> GPLGSGGGTIAMLNEISSDTLEQLYSLAFNQYQSGKYEDAHKVFQALCVLDHYDSRFFLGLGACRQAMGQYDLAIHSYSYGAVMDIKEPRFPFHAAECLLQKGELAEAESGLFLAQELIANKPEFKELSTRVSSMLEAIKLKKEMKHE;> XQVPELIKPSQ

SycD (specific Yop chaperone D) from the enteropathogen Yersinia enterocolitica is the class II chaperone of the translocator proteins YopD (Yersinia outer protein D) and YopB (Yersinia outer protein B). Like all known class II chaperones SycD exhibits an all α-helical structure. Six helices (H1A, H1B, H2A, H2B, H3A, H3B) fold into three tetratricopeptide repeats (TPRs), tandemly arranged motifs of some 34 amino acids length. The superhelical arrangement of tandem TPRs results in a curved structure with a convex outer surface and a concave inner side, which forms a mostly hydrophobic groove in T3S class II chaperones.

In order to verify that YopD binds to SycD via the proposed sequence motif 58PELIKP63 we co-crystallized N- and C-terminally truncated SycD21-163 with a synthetic peptide corresponding to YopD56-65 (56QVPELIKPSQ65). The chaperone peptide complex crystallized in the trigonal space group P3121 with one monomer per asymmetric unit. The Fo-Fc difference map clearly revealed positive electron density within the concave groove of SycD21-163, which allowed the easy positioning of the peptide residues 56’-64’ whereas Gln65’ could not be placed due to missing electron density. The peptide binds in an extended form into the chaperone’s hydrophobic cleft that is lined by aromatic and aliphatic residues from helix H1A and H2A. The antiparallel orientation relative to helix H1A allows the peptide’s hydrophobic residues Pro58’, Leu60’ and Pro63’ to perfectly fit into three distinct hydrophobic pockets within the concave groove whereas the charged residues Glu59’ and Lys62’ point outwards without contacting the chaperone. The pocket for Leu60’ of the peptide is exclusively hydrophobic and is mainly built by the SycD residues Phe44, Tyr47 (H1A), Phe59 (H1B), Leu74, Gly75 and Ala78 (H2A). The region of the concave groove that binds Pro58’ has a mixed hydrophobic and polar character and is formed by Tyr47 (H1A), Ala78 (H2A), Gln81 (H2A), Tyr93 (H2B) and His109 (H3A). Direct hydrogen bonds are formed between the hydroxyls of SycD Tyr40 and Tyr47 and the carbonyl oxygen of the peptide residues Ile61’ and Pro58’, respectively, and between the guanidino group of Arg146 (H8) and the side chain of Gln56’. The residues lining the concave groove do not show significant conformational changes between the apo and the peptide-bound form, suggesting a preformed and largely rigid binding site. The peptide’s three conserved anchor residues bind into distinct binding pockets within the concave region leading to a peptide conformation that is nearly identical to that of the CBDs of PopD and IpaB in complex with their respective chaperones.>[4x]GASRQRKLEALIRDPRSPINVESLLDGLNSLVLDLDFPALRKNKNIDNFLNRYEKIVKKIRGLQMKAEDYDVVKVIGRGAFGEVQLVRHKASQKVYAMKLLSKFEMIKRSDSAFFWEERDIMAFANSPWVVQLFYAFQDDRYLYMVMEYMPG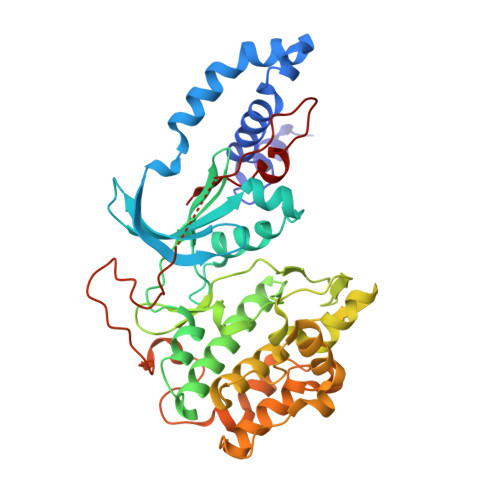GDLVNLMSNYDVPEKWAKFYTAEVVLALDAIHSMGLIHRDVKPDNMLLDKHGHLKLADFGTCMKMDETGMVHCDTAVGTPDYISPEVLKSQGGDGFYGRECDWWSVGVFLYEMLVGDTPFYADSLVGTYSKIMDHKNSLCFPEDAEISKHAKNLICAFLTDREVRLGRNGVEEIRQHPFFKNDQWHWDNIRETAAPVVPELSSDIDSSNFDDIEDDKGDVETFPIPKAFVGNQLPFIGFTYYR>[2x]MTTAPQEPPARPLQAGSGAGPAPGRAMRSTTLLALLALVLLYLVSGALVFRALEQPHEQQAQRELGEVREKFLRAHPCVSDQELGLLIKEVADALGGGADPETQSTSQSSHSAWDLGSAFFFSITIITTIGYGNVALRTDAGRLFCIFYALVGIPLFGILLA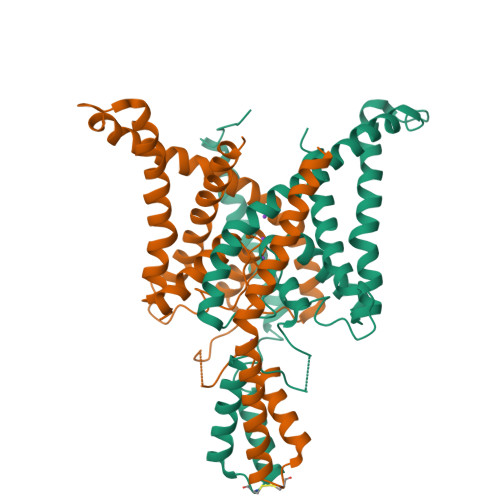GVGDRLGSSLRHGIGHIEAIFLKWHVPPELVRVLSAMLFLLIGCLLFVLTPTFVFCYMEDWSKLEAIYFVIVTLTTVGFGDYVAGADPRQDSPAYQPLVWFWILLGLAYFASVLTTIGNWLRVVSRRTRAEMGGLTAQSNSLEVLFQ>[2x]GADPFASITHLVDSAMVNKTDSIDREKTSDEPKPIEADESFDDFIYNFASDDALQRQRVVFPLPYYNGERASK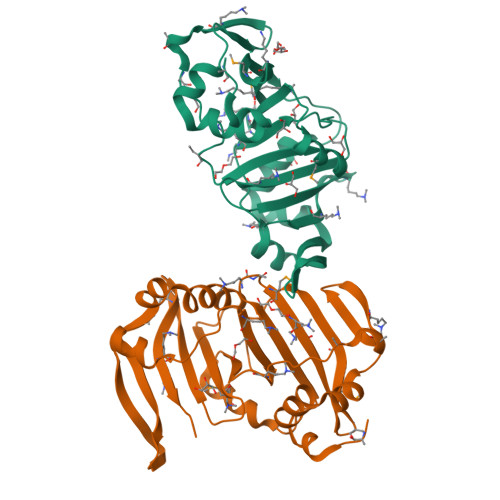IDRKYWKHDDLFAKQSYYTLLFDREEDMDLVGDTSLTSVQVEWIFVKKRMVKKYYFERIKGAWMLEAINLRPIEENENEDFVEFFGHFATDSIFQSRRIRQPLVFVTTDPDDDFSILETTLDLNQWFAFKPALPADKLSNINYGQQNDDNASHKILALKGIGNGFSNILYFQRKDSGWELYKFEDTSI>MANVEKMSVAVTPQQAAVMREAVEAGEYATASEIVREAVRDWLAKRELRHDDIRRLRQLWDEGKASGRPEPVDFDALRKEARQKLTEVPPNGR[2x];>[2x]MGSSHHHHHHSQDPMAVRLVWSPTAKADLIDIYVMIGSENIRAADRYYDQLEARALQLADQPRMGVRRPDIRPSARMLVEAPFVLLYETVPDTDDGP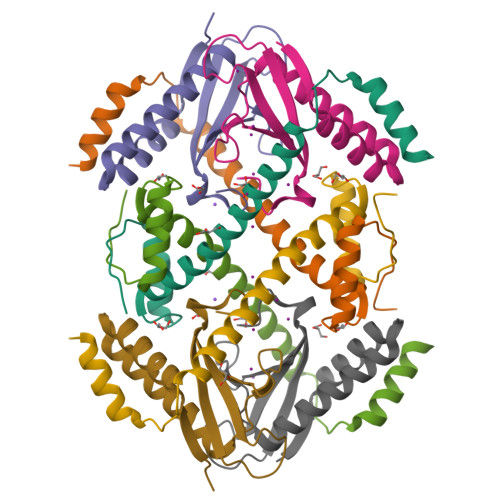VEWVEIVRVVDGRRDLNRLF> KELVLALYDYQEKSPRE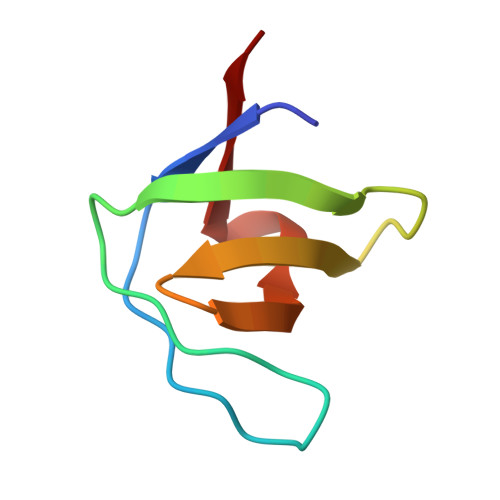VTMKKGDILTLLNSTNKDWWKVEVNGRQGFVPAAYVKKLD> MSGKGTSSRAYDMIMKLLLVGDSGVGKSCLLLRFVEDKFNPSFITTIGIDFKIR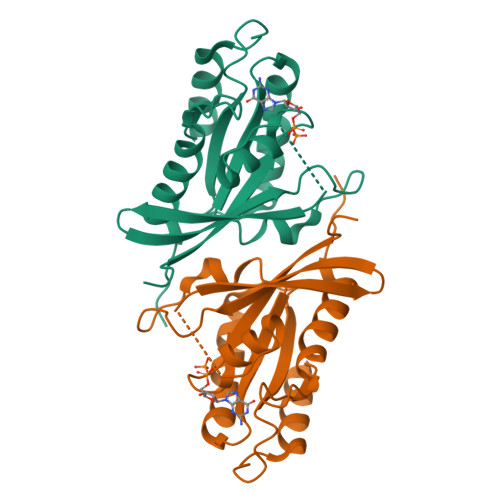TIESKGKRIKLQVWDTAGQERFRTITTAYYRGAMGIVLIYDVTDSRSFENVENWFQTVTQHANEDAQIFLVGNKCDDEVNRQVSKEQGQELAAKLNVPFLEASAKSNENVDSIFYELASIIQEKHVEENI N~2~-(2-cyano-5-methyl-1H-indole-7-sulfonyl)-N~2~-methyl-N-[4-(oxetan-3-yl)-3,4-dihydro-2H-1,4-benzoxazin-7-yl]glycinamide 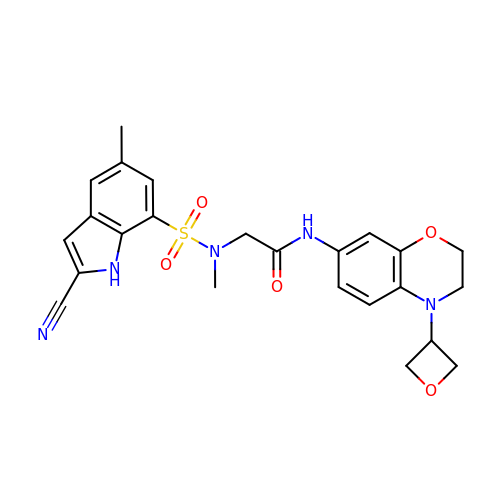| C24 H25 N5 O5 S | LICCSNABLLQTEJ-UHFFFAOYSA-N> MAENREPRGAVEAELDPVEYTLRKRLPSRLPRRPNDIYVNMKTDFKAQLARCQKLLDGGARGQNACSEIYIHGLGLAINRAINIALQLQAGSFGSLQVA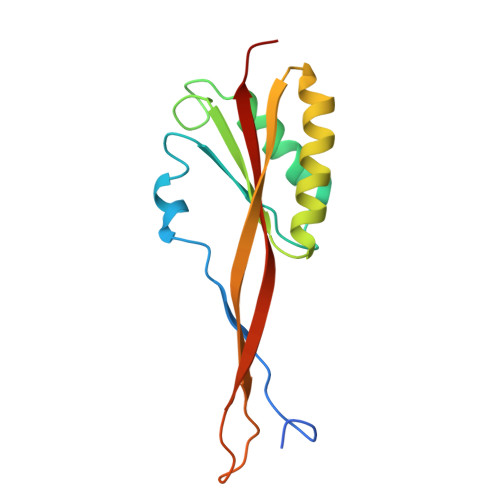ANTSTVELVDELEPETDTREPLTRIRNNSAIHIRVFRVTPK> MADSDINIKTGTTDIGSNTTVKTGDLVTYDKENGMHKKVFYSFIDDKNHNKKLLVIRTKGTIAGQYRVYSEEGANKSGLAWPSAFKVQLQLPDNEVAQISDYYPRNSIDTKEYMSTLTYGFNSNVTGDDTGKIGGLIGANVSIGHTLRYVQPDFKTILESPTDKKVGWKVIFNNMVNQNWGPYDRDSWNPVYGNQLFMKTRNGSMKAADNFLDPNKASSLLSSGFSPDFATVITMDRKASKQQTNIDVIYERVRDDYQLHWTSTNWKGTNTKDKWTDRSSERYKIDWEKEEMTNGSSGSVTTLSGLSGEQGPSGDMTTEEDSATHIKFSKRD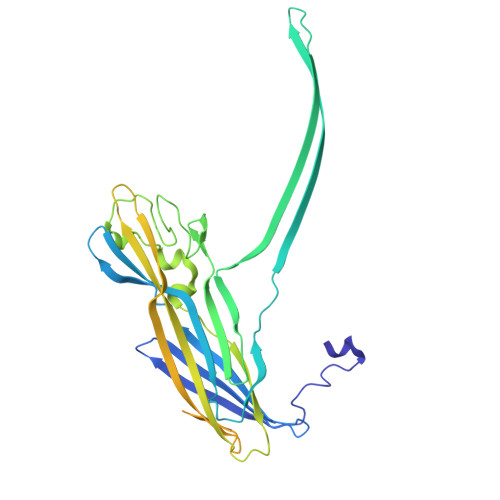EDGRELAGATMELRDSSGKTISTWISDGHVKDFYLYPGKYTFVETAAPDGYEVATPIEFTVNEDGQVTVDGEATEGDAHTGGSHHHHHH>MKRKIIYLASPYGFSQQQKTLLLPPIVRALEALGIEVWEPFARNNQIDFSQADWAYRVAQADLQDVKNCDGIFAVVNGTPPDEGVMVQLGMAIALNKAIFLFRDDFRRCSDNERYPLNLMLFAGLPEIGWENYYYTSVDEIQSHDKALYKWLTGM[3x];> MKRKIIYLASPYGFSQQQKTLLLPPIVRALEALGIEVWEPFARNNQIDFSQADWAYRVAQADLQDVKNCDGIFAVVNGTPPDEGVMVQLGMAIALNKAIFLFRDDFRRCSDNERYPLNLMLFAGLPEIGWENYYYTSVDEIQSHDKALYKWLTG

Here, we characterize the structure and function of a thermophilic dNDT, the protein from Chroococcidiopsis thermalis (CtNDT). Nucleoside 2′-deoxyribosyltransferase (dNDT) enzymes catalyze transglycosylation via a covalent 2′-deoxyribosylated enzyme intermediate with retention of configuration, having applications in the biocatalytic synthesis of 2′-deoxynucleoside analogues in a single step. The reaction catalyzed by dNDT proceeds via a ping-pong mechanism, with the formation of a 2′-deoxyribosyl-enzyme intermediate covalently linked to an active-site glutamate.13 Transglycosylation occurs in a stereospecific manner, preserving the anomeric carbon in the β configuration in the newly formed 2′-deoxyribonucleoside. As with other NDT enzymes, the active site of CtNDT is formed by residues from two monomers, and therefore, it is only fully formed in the dimer/tetramer.

By homology, E88 acts as a nucleophile, forming a glycosidic bond with the donor substrate. Our data show that CtNDTE88A is catalytic inactive, as expected, but CtNDTE88Q retains some catalytic activity, albeit the catalytic efficiency in comparison to the wild type is reduced by almost 50-fold. Any residual activity is unexpected given the crucial role proposed for E88 and might indicate that another residue in the active site vicinity can play a compensatory role in lieu of E88. This residue could be D62, as it is within hydrogen-bonding distance from the C1 of the sugar and E88 (kinetic parameters for mutants are given in Table S4and a discussion on the structure is given below). Enzyme–substrate complex (or enzyme–product complex, depending on the reaction direction): the complex CtNDTE88Q-clofarabine shows the 3′-OH of the arabinofuranosyl sugar within the hydrogen-bonding distance (3.3 Å) of S10. E88Q is 3.2 Å from C1′ in the sugar, 2.8 Å from Y7, and 3.3 Å from D62. E88Q and D62 are 3.3 Å apart, and therefore, Y7 can interact with either or both residues depending on the state in the reaction coordinate to ensure optimal positioning. Interactions with the nucleobase are mediated by hydrogen-bonding interactions with D111 and D62, and the 5′-OH is within the hydrogen-bonding distance of N118 (2.9 Å). The rate of 2′-deoxyribosylation was not significantly altered in E88Q-CtNDT compared with the WT enzyme, in agreement with covalent intermediate formation not being rate-limiting for kcat.>[2x]MAAQGPSPIPTNRLKQIAADACNDAIGSAEFYDHAKTEQWNHQIINTILKAVIAESQPSDSTTPPQFKFAVNSTIVQHLVPSSKLNKPAGGADDKPASTATSTDGKPHVGRRGMHSATGAFWNDKTDGMWTYKHEGDESKGMDVVVMLIWIAVLEHHHHHH;> AAPQNLTTVPLTTIYECPPSPVKEIFSYSKGIQTQ

Here we present the crystal structure of the protein encoded by MGG_01005, a gene that is important for vegetative mycelial growth of M. oryzae. Although there is only low sequence conservation with the Dynein light chain Tctex-type 1 (dynlt1/3), from yeast, human, mouse and fruit fly, the crystal structure of the gene product, MGG_01005, adopts the dynein light-chain Tctex-1 fold. Pull-down and yeast two-hybrid analysis demonstrate an interaction with the N-terminal region of the M. oryzae dynein intermediate chain (DIC) MoDyn1I2 as observed for other dynlt1/3 proteins confirming MGG_01005 as the dynlt1/3 of M. oryzae. Importantly, the structure of a complex of MGG_01005 with an N-terminal peptide from MoDyn1I2117–150 together with mutagenesis studies reveal that a di-histidine motif, widely conserved in dynlt1/3 proteins interacts with a highly conserved glutamate residue in the DIC.

Using this approach, and the apo-MGG_01005 structure as a search model, we were successful in solving an MGG_01005 - MoDyn1I2117–150 peptide complex structure by molecular replacement using PHASER implemented in the PHENIX platform (McCoy et al., Adams et al.). In the complex, there are two copies of MGG_01005 and one MoDyn1I2117–150 peptide per asymmetric unit. The rmsd after alignment of Cα positions of the A chains is 0.7 Å indicating that there is no large conformational change in MGG_01005 upon binding to the MoDyn1I2117–150 peptide. Notably, residues of 80–84 and 104–112, which could not be built in the model of apo structure, are present in chain A of the complex. In the first, residues of 122–141 of the MoDyn1I2117–150 peptide interact with a single MGG_01005 dimer within the ASU. Inspection of the protein-protein interface reveals that MGG_01005 mainly makes hydrophobic interactions and mainchain - mainchain hydrogen bonds with the MoDyn1I2117–150 peptide. Among these interactions, E138 makes a salt bridge with K139 of MoDyn1I2117–150 and the F121 side chain makes hydrophobic interactions with both the T124 main chain and V125 side chain of MoDyn1I2117–150. At the interface with MGG_01005 Monomer B there are seven hydrophobic interactions and one salt bridge, largely mediated by H34 and a conserved EXPP motif comprising residues 132–135 of MoDyn1I2117–150. Here, H34 makes both a salt bridge and a hydrophobic interaction with E132 of the motif whilst additionally the aliphatic portion of the chain E132 of MoDyn1I2117–150 also interacts with H115 of monomer A by a hydrophobic interaction. Nevertheless, taken together with the Y2H analysis these results reveal that while residues H34 and H115 are required for MoDyn1I2 binding, residues 80–112 are dispensable.> MTDTPFIRPDMKAFLEAIAAMAGPTLAEMTLEEARASYVALHGMADRPARELAVIRNLSCPGPAGDIPLRLYDARESREAGPVITFYHGGGFVIGDLDTHHNLCTEIAALMDLPVVAVDYRLAPEHPFPAAIEDCEAATRWVASSPSELGRTASGVIPIGDSAGGNATIVVSQLLGAKPADVPVVLQVPIFPLASDAVGSASLEAFAEGFVLTKASIEFFDTAYKADRADPRGFPILGDHTAAPPTIVATASLDPIR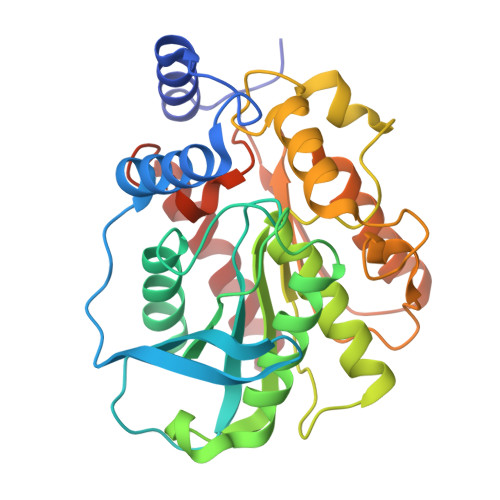DSGRDYAKALVEAGRDVVYLEMEGVTHSFTNIRAAVPSTQGDLERIIAAMKMMLGTA>MKMKLAVLPGDGIGPEVMDAAIRVLKTVLDNDGHEAVFENALIGGAAIDEAGTPLPEETLDICRRSDAILLGAVGGPKWDHNPASLRPEKGLLGLRKEMGLFANLRPVKAYATLLNASPLKRERVENVDLVIVRELTGGLYFGRPSERRGPGENEVVDTLAYTREEIERIIEKAFQLAQIRRKKLASVDKANVLESSRMWREIAEETAKKYPDVELSHMLVDSTSMQLIANPGQFDVIVTENMFGDILSDEASVITGSLGMLPSASLRSDRFGMYEPVHGSAPDIAGQGKANPLGTVLSAALMLRYSFGL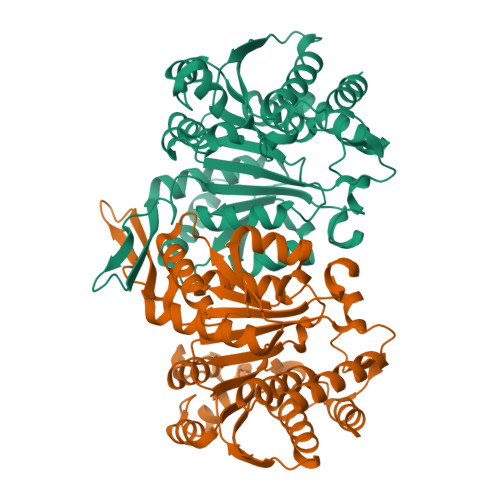EKEAAAIEKAVDDVLQDGYCTGDLQVANGKVVSTIELTDRLIEKLNNSAAGPRIFQ[2x]> MLSRRLVRAVAPLRSPVLPAARRLPLIQQRTFLPEAMVGRSKIDEKYPDSDYPTLTDKEDPDMNGGYINPPRIKRQFRDPHADWWDKQERRNFGEPVHEDHDILGMFSPYEYTWITPGKGLFQIGLFIASFLGLCYVVKLTYPDRVSYPREFEGGLERELGGAGAVRAFLCLDDEIMW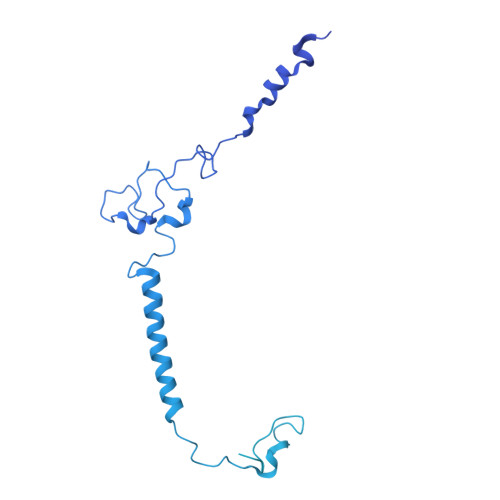MVSLYCLPASKLISSPVALQDKSTSSASAMRYDDWDVILFPTGRDSKIPFKEFKVACHVVPDIELAHLHGAVGSPVMTCFVPSLPPGTPFQVSIHCWRRPEISQFARTYSKNPDLVKFEARVTLDGRLVASAILDRDVNGPHLITSTFEFTKTGELERLTFPAFRQEILRQNHWHPGDDLGRIKVIISEGFPRDSLTVPIERVKNIVTFSFQHAPLGKIPGIAWPNPGMWRRPTPNPAVSVPTYFPGDGAESHAHSPGKRSLLLKGIRNHGFPSTVIPGSIFHHQSNPAGLLNPPGFKVPHFSASNPSVPNIFSPHDPFAEPTYRDWMSSITNVQAGDFWDGRTTWPINPRNFHKSDTIMADCPSQGGDPMQISGSSLEDDPLRLKAPQNTPTEGGEGPNPGAQFAHPIPSELTADLESALSQSLLNQAPTSAISQRNFPMPHSDGLSRKEGRQVSLGQGTSAQMPSTSSSMEARRLSQALFGMNNLPIEASVNNGVSASVTPLFAANQRSVNNPLVATFGSAILSQGSTNPSGTEQSTDTTATTTAAAAAAVTDVQVEPPAPTSNAANESVINLTSGTSSTSTVHANVPTSVSKRPRNFTPASARVIDEEDEPRRTSPQVQVGGFAETTSVEESIQ>MFQQLSARLQEAIGRLRGRGRITEEDLKATLREIRRALMDADVNLEVARDFVERVREEALGKQVLESLTPAEVILATVYEALKEALGGEARLPVLKDRNLWFLVGLQGSGKTTTAAKLALYYKGKGRRPLLVAADTQRPAAREQLRLLGEKVGVPVLEVMDGESPESIRRRV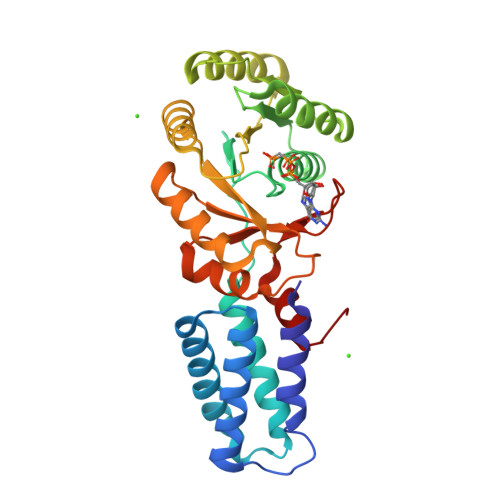EEKARLEARDLILVDTAGRLQIDEPLMGELARLKEVLGPDEVLLVLDAMTGQEALSVARAFDEKVGVTGLVLTKLDGDARGGAALSARHVTGKPIYFAGVSEKPEGLEPFYPERLAGRILGMGDV[2x]Bacteriophage T5, a representative member of the T5-like family of siphophages, serves as an excellent model for studying the assembly, infection, cell wall perforation, and DNA ejection mechanisms of this phage family. In this study, we used cryo-electron microscopy (cryo-EM) to determine the structures of mature T5 (a laboratory-adapted, fiberless T5 mutant) and urea-treated empty T5 (lacking the tip complex) at near-atomic resolutions. The T5 head comprises 775 copies of MCP gp8, arranged into 11 pentons and 120 hexons, forming an icosahedral shell with a triangle number (T) of 13. The T5 tail, which comprises 40 trimeric rings of the TTP and a distal tip complex, is connected to a unique five-fold vertex of the head by the connector complex.

We built atomic models for the portal, adaptor, and tail terminator of urea-treated empty T5. In contrast to the mature T5, the DNA and TMP are ejected in urea-treated empty T5, resulting in an empty head and an unoccupied tail tube. The tail terminator comprises six copies of protein p142. Each p142 contains two α-helices and a β-barrel structure facing the lumen of the tube, which are homologous to the terminator proteins of other phages, such as Lambda (gpU) and SPP1 (gp17). Structural comparisons of the portal, adaptor, and tail terminator proteins before and after DNA release indicated that no discernible conformational changes had occurred in these regions during infection. In the mature state, the negative electrostatic potential inside the connector channel and TMP collectively prevent the release of DNA. In the DNA-ejected state, once the interaction of the tail tip complex or baseplate with the host cell induces the release of TMP, the large space of the connector complex enables the passage of DNA. Therefore, the connector complex may not be directly involved in the aforementioned processes. Notably, the tip complex of the empty particle became detached for urea-treatment-induced reasons.

>[6x]MDHRTSIAQAMVDRISKQMDGSQPDEYFNNLYGNVSRQTYKFEEIREFPYVAVHIGTETGQYLPSGQQWMFLELPILVYDKEKTDIQEQLEKLVADIKTVIDTGGNLEYTVSKPNGSTFPCEATDMIITSVSTDEGLLAPYGLAEINVTVRYQPPRRSLRR> MDYKDDDDKGVPRIPMASVASCDSRPSSDELPGDPSSQEEDEDYDFEDRVSDSGSYSSASSDYDDLEPEWLDSVQKNGELFYLELSEDEEESLLPETPTVNHVRFSENEIIIEDDYKERKKYEPKLKQFTKILRRKRLLPKRCNKKNSNDNGPVSILKHQSNQKTGVIVQQRYKDVNVYVNPKKLTVIKAKEQLKLLEVLVGIIHQTKWSWRRTGKQGDGERLVVHGLLPGGSAMKSG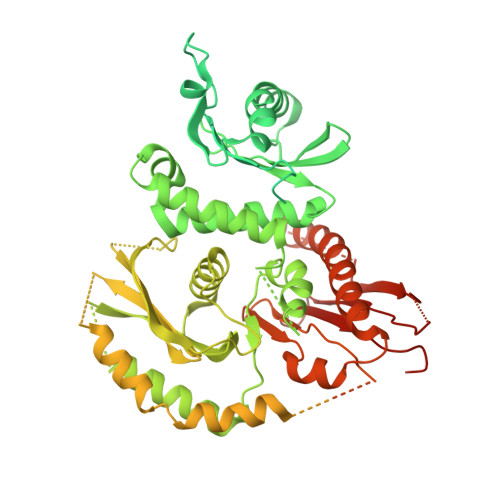QVLIGDVLVAVNDVDVTTENIERVLSCIPGPMQVKLTFENAYDVKRETSHPRQKKTQSNTSDLVKLLWGEEVEGIQQSGLNTPHIIMYLTLQLDSETSKEEQEILYHYPMSEASQKLKSVRGIFLTLCDMLENVTGTQVTSSSLLLNGKQIHVAYWKESDKLLLIGLPAEEVPLPRLRNMIENVIQTLKFMYGSLDSAFCQIENVPRLDHFFNLFFQRALQPAKLHSSASPSAQQYDASSAVLLDNLPGVRWLTLPLEIKMELDMALSDLEAADFAELSEDYYDMRRLYTILGSSLFYKGYLICSHLPKDDLIDIAVYCRHYCLLPLAAKQRIGQLIIWREVFPQHHLRPLADSSTEVFPEPEGRYFLLVVGLKHYMLCVLLEAGGCASKAIGSPGPDCVYVDQVKTTLHQLDGVDSRIDERLASSPVPCLSCADWFLTGSREKTDSLTTSPILSRLQGTSKVATSPTCRRTLFGDYSLKTRKPSPSCSSGGSDNGCEGGEDDGFSPHTTPDAVRKQRESQGSDGLEESGTLLKVTKKKSTLPNPFHLGNLKKDLPEKELEIYNTVKLTSGPENTLFHYVALETVQGIFITPTLEEVAQLSGSIHPQLIKNFHQCCLSIRAVFQQTLVEEKKKGLNSGDHSDSAKSVSSLNPVKEHGVLFECSPGNWTDQKKAPPVMAYWVVGRLFLHPKPQELYVCFHDSVTEIAIEIAFKLFFGLTL>MENLISLVNKIQRACTALGDHGDSSALPTLWDSLPAIAVVGGQSSGKSSVLESIVGKDFLPRGSGIVTRRPLVLQLQKIDDGTREYAEFLHLPRKKFTDFAAVRKEIQDETDRETGRSKAISSVPIHLSIYSPNVVNLTLIDLPGLTKVAVDGQSDSIVKDIENMVRSYIEKPNCIILAISPANQDLATSDAIKISREVDPSGDRTFGVLTKIDLMDKGTDAVEILEGRSFKLKYPWVGVVNRSQADINKNVDMIAARKREREYFSNTTEY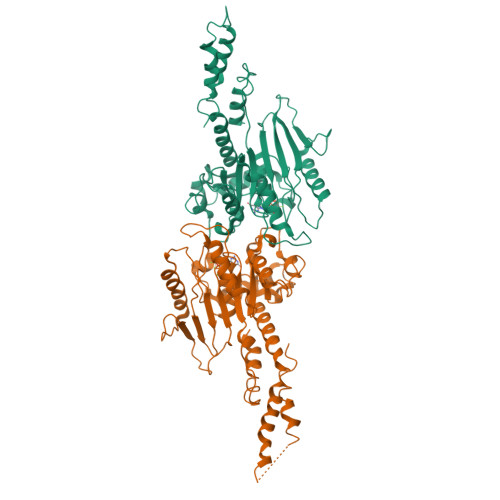RHLANKMGSEHLAKMLSKHLERVIKSRIPGIQSLINKTVLELETELSRLGKPIAHGTDSRVDPAIMERRSAISKRLELYRAAQSEIDAV[2x]>[2x]MVLYFIGLGLYDERDITVKGLEIAKKCDYVFAEFYTSLMAGTTLGRIQKLIGKEIRVLSREDVELNFENIVLPLAKENDVAFLTPGDPLVATTHAELRIRAKRAGVESYVIHAPSIYSAVGITGLHIYKFGKSATVAYPKGNWFPTSYYDVIKENAERGLHTLLFLDIKAEKRMYMTANEAMELLLKVEDMKKGGVF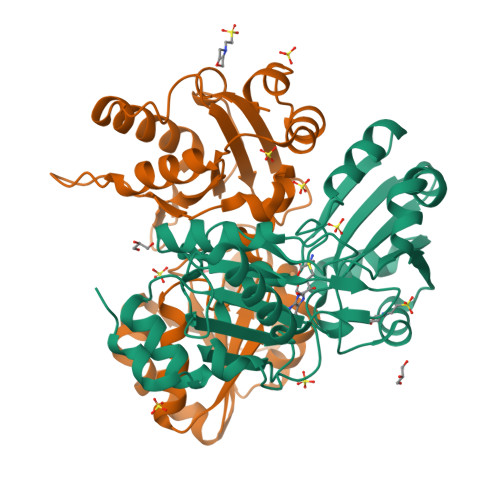TDDTLVVVLARAGSLNPTIRAGYVKDLIREDFGDPPHILIVPGKLHIVEAEYLVEIAGAPREILRVNV>MEKYNPHAIEAKWQRFWEEKGFMKAKDLPGGRGKQYVLVMFPYPSGDLHMGHLKNYTMGDVLARFRRMQGYEVLHPMGWDAFGLPAENAALKFGVHPKDWTYANIRQAKESLRLMGILYDWDREVTTCEPEYYRWNQWIFLKMWEKGLAYRAKGLVNWCPKCQTVLANEQVVEGRCWRHEDTPVEKRELEQWYLRITAYAERLLKDLEGLNWPEKVKAMQRAWIGRSEGAEILFPVEGKEVRIPVFTTRPDTLFGATFLVLAPEHPLTLELAAPEKREEVLAYVEAAKRKTEIERQAEGREKTGVFLGAYALNPATGERIPIWTADYVLFGYGTGAIMAVPAHDQRDYEFARKFGLPIKKVIERPGEPLPEPLERAYEEPGIMVNSGPFDGTESEEGKRKVIAWLEEKGLGKGRVTYRLRDWLISRQRYWGTPIPMVHCEACGVVPVPEEELPVLLPDLKDVEDIRPKGKSPLEAHPEFYETTCPKCGGPAKRDTDTMDTFFDSSWYYLRYTDPHNDRLPFDPEKANAWMPVDQYIGGVEHAVLHLLYSRFFTKFLHDLGMVKVEEPFQGLFTQGMVLAWTDFGPVEVEGSVVRLPEPTRIRLEIPESALSLEDVRKMGAELRPHEDGTLHLWKPAVMSKSKGNGVMVGPFVKEQGADIARITILFAAPPENEMVWTEEGVQGAWRFLNRIYRRVAEDREALLETSGVFQAEALEGKDRELYGKLHETLKKVTEDLEALRFNTAIAALMEFLNALYEYRKDRPVTPVYRTAIRYYLQMLFPFAPHLAEELWHWFWPDSLFEAGWPELDEKALEKDVVEVAVQVNGRVRGTIHIPKDAPLEVARAEALKVRNVRAHLEGKEVVKE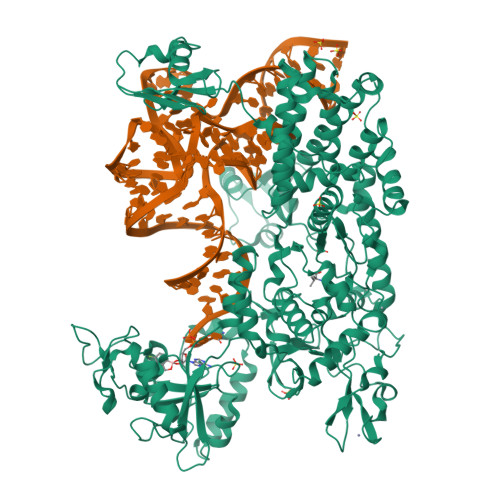IYVPGKILNLVVRG[2x]A widely applicable approach is the use of photocaged substrates, where the photocage is soaked into the crystal in advance and then activated using a laser pulse to provide uniform initiation of the reaction throughout the crystal. This work characterizes photocage release of nitric oxide and binding of this ligand to two heme protein systems, cytochrome c′-β and dye-decolourizing peroxidase B using a fixed target sample delivery system. In this work, we describe a thorough characterization of the application of the NO photocage N,N′-bis-(carb­oxy­methyl)-N,N′-di­nitroso-1,4-phenyl­enedi­amine (henceforth referred to as NO cage) to room-temperature microcrystals of two proteins: a gas binding cytochrome c′ (McCP-β) and a dye-decolourizing peroxidase B (DtpB). Laser parameters for photoactivation are systematically explored, and time-resolved structures over timescales ranging from 100 µs to 1.4 s using synchrotron and XFEL beamlines are described. We have demonstrated a sample and time efficient approach using fixed targets to carry out time-resolved SSX and SFX experiments with an NO photocage over the microsecond to second time regimes.

On binding to the heme, NO was observed to bind in an end-on fashion via the nitro­gen atom with an Fe—N distance of approximately 2.0–2.5 Å and an Fe—N—O angle of approximately 105–150°. The variability in these values occurs across the six independent heme groups within the crystallographic model and could represent either genuine differences in binding due to subtle differences in the crystalline environments or simply uncertainty in modelling a small ligand into the electron density features. A small shift in the side-chain position of Asn245 was observed compared with the ‘empty’ site structure in all six of the hemes, and at all laser powers and timepoints. An intriguing observation was that of differing occupancies for the released NO within the different (chemically identical) monomers of the homo-oligomeric proteins, particularly for the hexameric DtpB (in contrast, McCP-β is a homodimer). One possible explanation would be differences in the proximity to the bulk solvent channels in which the photocage molecules presumably are present, although no correlation was seen between chains with higher NO occupancy between the differing laser powers. Assessment of occupancies in light-activated processes remains challenging, particularly for small ligands such as the diatomic NO. For our experiments with DtpB, we found both B-factor and Fo − Fc peak height quantification to give results that display the same occupancy trend with laser power, but both generally overestimate NO occupancy compared with multicopy refinement [Fig. 6(f) and Table S4]. For DtpB, the structure of the NO ferric heme complex of this or any other B-type DyP have not been previously determined, and thus we have demonstrated here that such a complex rapidly forms on exposure to NO after photocage release.

>[6x]MWRYESVVGGCSFMGGEVEEPEPQMVLSPLTSAAIFLVVTIDSGGEDTVRDLLSDVASLERAVGFRAQPDGRLSCVTGIGSEAWDRLFSGARPAGLHPFRELDGPVHRAVATPGDLLFHIRASRLDLCFALATEIMGRLRGAVTPQDEVHGFKYFDERDMLGFVDGTENPTGAAARRAVLVGAEDPAFAGGSYAVVQKYLHDIDAWEGLSVEAQERVIGRRKMTDVELSDDVKPADSHVALTSVTGPDGSDLEILRDNMPFGSVGREEFGTYFIGYARTPEVTETMLERMFLGTASAPHDRILDFSTAVTGSLFFTPAADFLEDLSARP> APAVADKADNAFMMICTALVLFMTIPGIALFYGGLIRGKNVLSMLTQVTVTFALVCILWVVYGYSLAFGEGNNFFGNINWLMLKNIELTAVMGSIYQYIHVAFQGSFACITVGLIVGALAERIRFSAVLIFVVVWLTLSYIPIAHMVWGGGLLASHGALDFAGGTVVHINAAIAGLVGAYLIGKRVGFGKEAFKPHNLPMVFTGTAILYIGWFGANAGSAGT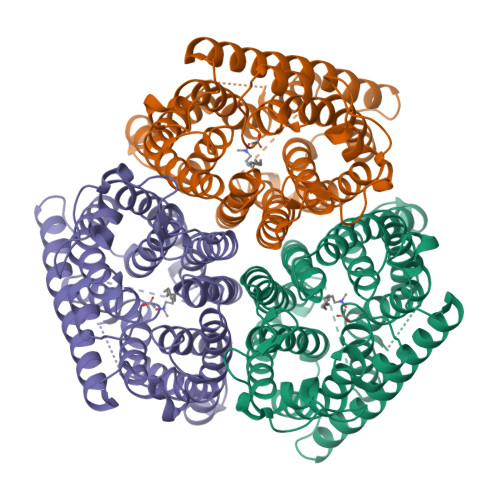ANEIAALAFVNTVVATAAAILGWIFGEWALRGKPSLLGACSGAIAGLVGVTPACGYIGVGGALIIGVVAGLAGLWGVTMLKRLLRVDDPCDVFGVHGVCGIVGCIMTGIFAASSLGGVGFAEGVTMGHQLLVQLESIAITIVWSGVVAFIGYKLADLTVGLRVPEEQEREGLDVNSHGENAYNADQAQQPAQADLEHHHHHH>[21x]MKMASTRCKLAR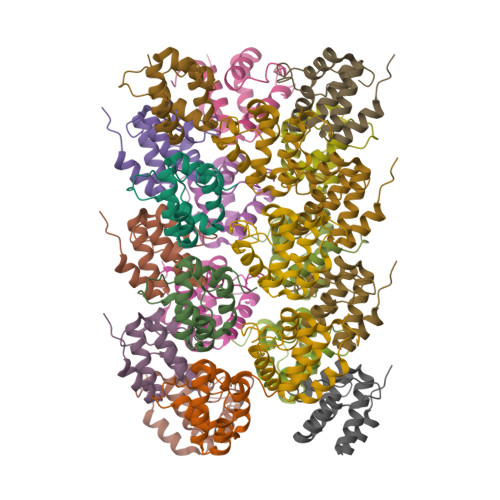YLEDLEDVDLKKFKMHLEDYPPQKGCIPLPRGQTEKADHVDLATLMIDFNGEEKAWAMAVWIFAAINRRDLYEKAKRDEPKWG> SREEFEQILQERNELKAKVFLLKEELAYFQRELLT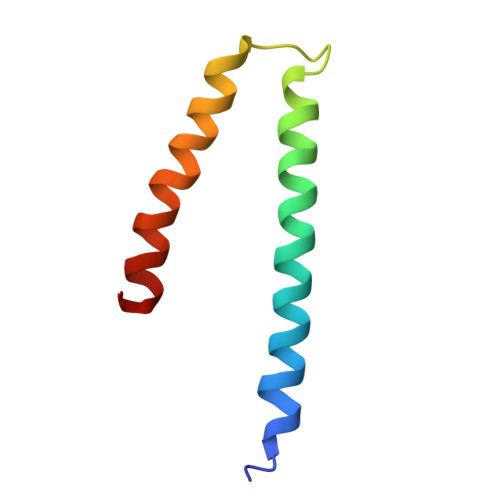DHRVPSLLLEAMKVAVRKQRKKIKAKMLGT>MNTIHHHHHNTSGSGGGGGRLVPRGSMSENLYFQGSMSKNNIFNKYPTIIHGEARGENDEFVVHTRYPRFLARKSFDDNFTGEMPAKPVNGELGQIGEPRRLAYDSRLGLWLSDFIMLDNNKPKNMEDWLGQLKAACDRIAADDLMLNEDAADLEGWDD[2x]

In this work, we investigate the mechanism of activity of anti-CRISPR protein AcrIIC2Nme. This 123-residue protein was previously shown to inhibit the activity of Neisseria meningitidis CRISPR-Cas9 in vivo and in vitro. We show that AcrIIC2Nme functions by inhibiting loading of the guide RNA molecule, thereby preventing formation of the active CRISPR-Cas9 surveillance complex. We found that it blocks Cas9 binding to sgRNA, thereby inhibiting biogenesis of the surveillance complex. This interference is mediated through an interaction with the arginine-rich bridge helix, which connects the REC lobe to the NUC lobe.

To better understand the precise mechanism by which AcrIIC2Nme inhibits Cas9 activity, we determined its crystal structure to a resolution of 2.5 Å using single-wavelength anomalous diffraction (SAD). Consistent with these previous observations, AcrIIC2Nme shares no sequence or structural similarity with previously characterized anti-CRISPR proteins. We also created a mutant lacking the final 12 amino acids (Δ112–123), which were not resolved in one of the apo crystal structures. The crystal structure of AcrIIC2Nme revealed a highly negatively charged surface that binds to the positively charged bridge helix. Mutation of this electronegative surface decreases the affinity of AcrIIC2Nme for Cas9, resulting in loss of anti-CRISPR activity. To determine if the interactions between AcrIIC2Nme and the bridge helix of Nme1Cas9 are required and sufficient for anti-CRISPR inhibitory activity, we mutated 19 residues distributed widely across the surface of AcrIIC2Nme. Mutation of three of the four amino acids that make direct contacts with the bridge helix (E17A, E24A, D108A) displayed a complete lack of anti-CRISPR activity in vivo while the other mutants showed changes in activity of less than 10-fold. Circular dichroism spectroscopy of the three mutants with abrogated in vivo activity revealed spectra similar to the wild type protein, showing that the lack of activity was not due to a folding defect. In addition, cooperative thermal denaturation curves and melting temperatures similar to the wild type protein indicated that these mutants maintained stable, folded structures. We conclude that the negatively charged surface of AcrIIC2Nme and the positively charged Nme1Cas9 bridge helix comprise a critical interaction interface that is required for anti-CRISPR activity.> CIDGKAKIIFENEGEEHLTTMEEMYERYKHLGEFYDEEYNRWGIDVSNVPIYVKSFDPESKRVVKGKVNVIWKYELGKDVTKYEIITNKGTKILTSPWHPFFVLTPDFKIVEKRADELKEGDILIGGMPDGEDYKFIFDYWLAGFIAGDGCFDKYHSHVKGHEYIYDRLRIYDYRIETFEIINDYLEKTFGRKYSIQKDRNIYYIDIKARNITSHYLKLLEGIDNGIPPQILKEGKNAVLSFIAGLFDAEGHVSNKPGIELGMVNKRLIEDVTHYLNALGIKARIREKLRKDGIDYVLHVEEYSSL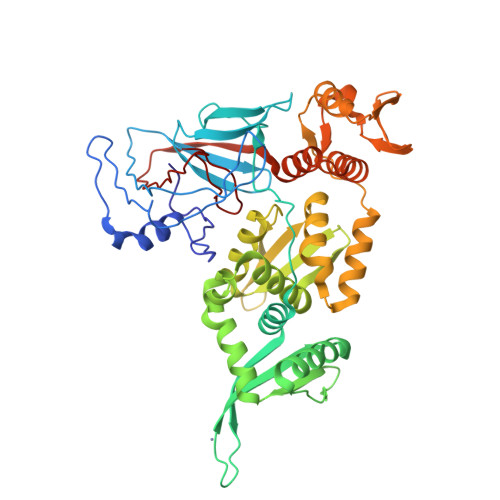LRFYELIGKNLQNEEKREKLEKVLSNHKGGNFGLPLNFNAFKEWASEYGVEFKTNGSQTIAIINDERISLGQWHTRNRVSKAVLVKMLRKLYEATKDEEVKRMLHLIEGLEVVRHITTTNEPRTFYDLTVENYQNYLAGENGMIFVHN>SIGTRWAVLIAGSKGYHNYRHQADVCHMYQILRKGGVKDENIIVFMYDDIAYNESNPFPGIIINKPGGENVYKG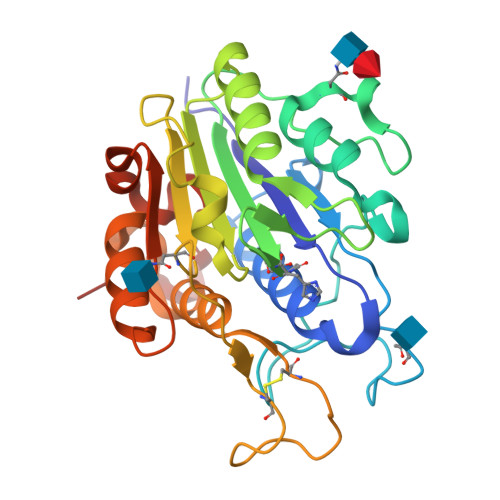VPKDYTGEDINNVNFLAAILGNKSAIIGGSGKVLDTSPNDHIFIYYAXGAPGKIGMPSKPYLYADDLVDTLKQKAATGTYKSMVFYVEAANAGSMFEGLLPEGTNIYAMAASNSTEGSWITYCPGTPDFPPEFDVCLGDLWSITFLEDCDAHNLRTETVHQQFELVKKKIAYASTVSQYGDIPISKDSLSVYMGTDPANDNRTFVDEN[2x]>[6x]MSKSDVFHLGLTKNDLQGAQLAIVPGDPERVEKIAALMDKPVKLASHREFTSWRAELDGKAVIVCSTGIGGPSTSIAVEELAQLGIRTFLRIGTTGAIQPHINVGDVLVTTASVRLDGASLHFAPMEFPAVADFACTTALVEAAKSIGATTHVGVTASSDTFYPGQERYDTYSGRVVR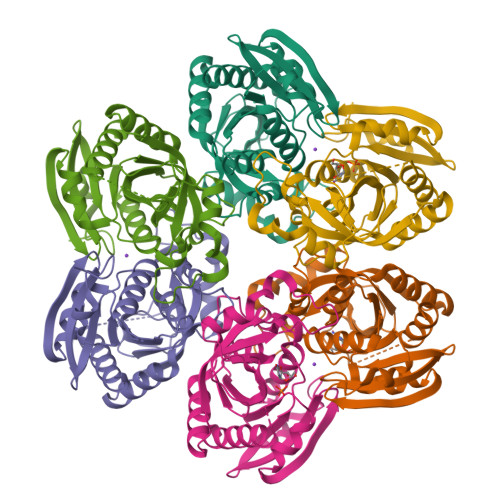RFKGSMEEWQAMGVMNYEMESATLLTMCASQGLRAGMVAGVIVNRTQQEIPNAETMKQTESHAVKIVVEAARRLL>MGAFTGKTVLILGGSRGIGAAIVRRFVTDGANVRFTYAGSKDAAKRLAQETGATAVFTDSADRDAVIDVVRKSGALDILVVNAGIGVFGEALELNADDIDRLFKINIHAPYHASVEAARQMPEGGRILIIGSVNGDRMPVAGMAAYAASKSALQGMARGLARDFGPRGITINVVQPGPIDTDANPANGPMRDMLHSLMAIKRHGQPEEVAGMVAWLAGPEASFVTGAMHTIDGAFGAL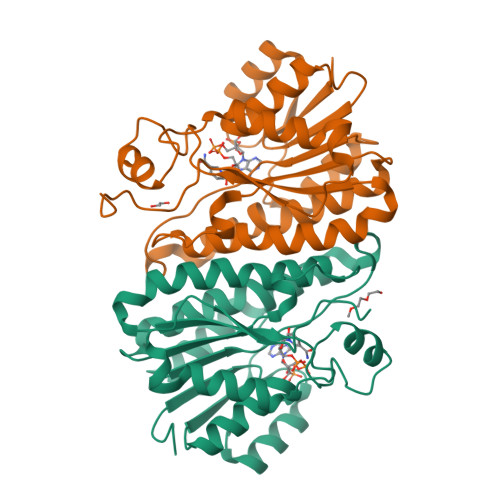EHHHHHH[12x]>MNNRNHDVLSRMISEKAALHGLLNCLIKEFAIPEGYLRYEWPDEMKGIPPGAYFDGADWKGIPMMIGLPDQLQLFVMVDRRDTFGSQHYLSDVYLRQAQGDWQCPDFEPLVARLLAACEHIAGRKNPELYEQILQSQRLVSAIVSHNGRQRADAPLQHYLQSEQGLWFGHPSHPAPKARLWPAHLGQEQWAPEFQARAALHQFEVPVDGLHIGANGLTPQQVLDGFADQQPASPGHAIICMHPVQAQLFMQDARVQQLLRDNVIRDLGQSGRVASPTASIRTWFIDDHDYFIKGSLNVRITNCVRKNAWYELESTVLIDRLFRQLLDQHADTLGGLVAAAEPGVVSWSPAAAGELDSHWFREQTGGILRENFCRRTGAERSIMAGTLFARGVDLQPMIQTFLRTHYGEALDDNALLYWFDDYQTRLLRPVLSLFFNHGVVMEPHLQNSVLVHQQGRPQQVLLRDFEGVKLTDDLGIRYIDDDIHPRVRQSLLYSREQGWNRIMYCLFINHLSETILALSQGRPQLAPLMWRRVQQQLRAIQGELKQPSPELDALIAGHPVACKTNLKVRLAAEADRQASYVRLPSPWGHAVQHGSEVQHDERRHGDVRHEEARHGEVQHG[2x]

The first NIS synthetase to be structurally characterized was the achromobactin biosynthesis protein D (AcsD), from the plant pathogen Dickeya dadantii (formally known as Pectobacterium chrysanthemi). AcsD catalyses the enantioselective desymmetrization of citric acid via adenylation of its pro-R carboxyl group with ATP. The resulting enzyme-bound homochiral citryl adenylate reacts with l-serine to generate the first committed intermediate, (3′S)-O-citryl-l-serine, in achromobactin biosynthesis. Structural and biochemical studies have characterized the first step of the reaction in detail. These showed that AcsD is a new member of the adenylating enzyme superfamily, with no sequence or structural homology to other members of the family.

However, growing crystals of AcsD pre-incubated with ATP, Mg2+, and ethylenediamine showed clear additional electron density for a molecule larger than citric acid in one subunit as well as density for ATP and Mg2+. We interpret this density as (3′S)-N-citryl-ethylenediamine (CEDA) and were able to refine the co-complex. ATP, Mg2+, the protein, and much of the citryl moiety of CEDA are in the same positions they have been previously observed to occupy in other co-complexes. The difference in position between the citryl moiety of CEDA and citrate in the previously reported citrate/adenosine/sulfate complex occurs in the regions occupied by the carboxamide group in CEDA (this work) and the pro-R carboxyl group of citrate (previous structure). The carboxamide group adopts a rotamer different from that of the citrate carboxyl group. If the carboxamide group did not do this, the ethylenediamine moiety would clash with the α-phosphate of ATP (and AMP). The ethylenediamine moiety of CEDA sits in a shallow cleft and makes several contacts with the protein. There is a particularly striking bidentate hydrogen bond interaction between both nitrogen atoms of CEDA and the two oxygen atoms of the side chain of E442. The side chains of R501 and K563 point towards the ethylenediamine moiety. Structural data show that AcsD uses E442 to achieve this recognition by making a striking bidentate interaction with CEDA.> AERSELTIHPKEFTTFVRNFNPFLGATNLHTTTDFIYEPLVVFNEMHGNTPVFRLA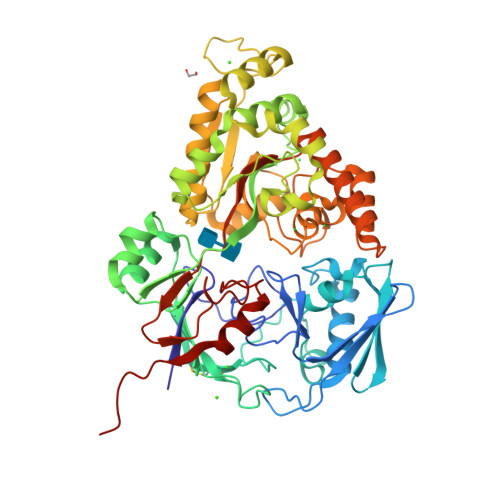ENFQMSDDLMSVTFDIRKGVKWSDGEAFTADDVVYSFNLVKEKPELDQSGINSWVTGVEKVNDYQVKFRLSEANSNVPYEIAKVPVVPKHVWSKVKDPSTFTNENPVGSGPFTVIDTFTPQLYIQCENPNYWDAANLDVDCLRVPQIANNDQFLGKVVNGEMDWTSSFVPDIDRTYAAASPKHHYWYPPAGTQAFVVNFKNPDAAKNEALTNVDFRRAFSMALDRQTIIDIAFYGGGTVNDFASGLGYAFEAWSDEKTHDKFKAYNSYNAEGAKKLLAKAGFKDVNKDGFVDTPSGKSFELLIQSPNGWTDFNNTVQLAVEQLAEVGIKARARTPDFSVYNQAMLEGTYDVAYTNYFHGADPYTYWNSAYNSALQSGDGMPRAAMHFYKNEKLDGLLNSFYKTADKQEQLEIAHGIQQIIAQDQVTIPVLSGAYMYQYNTTRFTGWWNEENPKGRPNIWAGIPERLLHVLDLKPVKLEHHHHHH>MVVKFTDSQIQHLMEYGDNDWSEAEFEDAAARDKEFSSQFSKLKSANDKGLKDVIANPRNDLTDLENKIREKLAARGFIEVHTPIF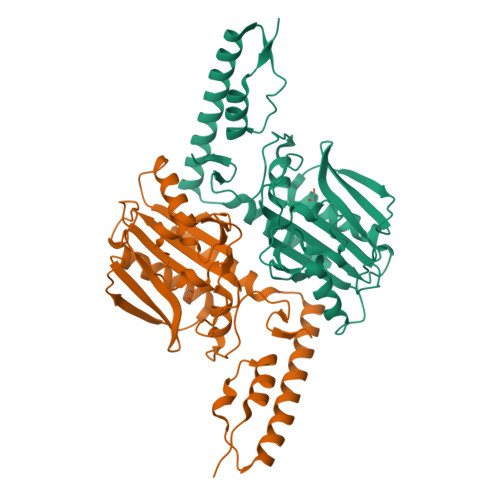VSKSALAKMTITEDHPLFKQVFWIDDKRALRPMHAMNALKVMRELRDHTKGPVKIFEIGSCFRKESKSSTHLEEFTMLNLAEMGPDGDPMEHLKMYIGDIMDAVGVEYTTSREESDVWVETLDVEINGTEVASGSVGPHKLDPAHDVHEPWAGIGFGLERLLMLKNGKSNARKTGKSITYLNGYKLD[4x]> MSDTNYAVIYDLHSHTTASDGCLTPEALVHRAVEMRVGTLAITDHDTTAAIAPAREEISRSGLALNLIPGVEISTVWENHEIHIVGLNIDITHPLMCEFLAQQTERRNQRAQLIAERLEKAQIPGALEGAQRLAQGGAVTRGHFARFLVECGKASSMADVFKKYLARGKTGYVPPQWCTIEQAIDVIHHSGGKAVLAHPGRYNLSAKWLKRLVAHFAEHHGDAMEVAQCQQSPNERTQLAALARQHHLWASQGSDFHQPCPWIELGRKLWLPAGVEGVWQLWEQPQNTTEREL

RNase AM is so far the only 5′-3′ exoribonuclease known in E. coli, the enzymatic activity of which has been shown to be essential for the processing of bacterial ribosomal RNA. RNase AM belongs to the PHP domain family of proteins which is composed of amidohydrolases/phosphoesterases and is present in some DNA polymerases. To test this, we assessed the deFADding and deNADding activities of a recently characterized 5′-3′ exoribonuclease in E. coli, RNase AM (yciV), which can hydrolyze short RNAs of up to five nucleotides with a 5′P. We were able to expand on the original observations and demonstrate that a 40 nucleotide RNA molecule can also be degraded by RNase AM and further demonstrate the exonuclease activity is processive. Intriguingly, RNase AM also demonstrated robust deFADding activity, but unlike the two eukaryotic nucleases, RNase AM did not hydrolyze NAD-capped RNA.

To gain insight into how an exoribonuclease could function as a deFADding enzyme, we attempted to determine the crystal structure of E. coli RNase AM in complex with FAD in an effort to elucidate the mechanism for RNase AM monophosphate hydrolysis and deFADding activities. However, no crystals were obtained for RNase AM alone or in the presence of FAD. No density for the RNase AM insertion domain was observed, indicating that the domain is disordered in this crystal. The final structure consists of residues 9–106 and 177–284 and is modeled with three manganese ions (Mnα, Mnβ, and Mnγ) and a sulfate molecule in the active site. The refined atomic model contained no RNA and has excellent agreement with the X-ray diffraction data and the expected bond lengths, bond angles and other geometric parameters. RNase AM has a distorted (β/α)7-barrel fold and a three metal enzyme active site composed of histidines and aspartates/glutamate residues. Mnα and Mnβ, which are proposed to coordinate the water for nucleophilic attack are coordinated by residues His13, Glu72 and Asp255, and Glu72, His83 and His198 respectively. Mnγ is coordinated by residues Asp20, His45 and His257. The sulfate molecule coordinates all three metals and forms a salt bridge with Arg201, which may stabilize the hydrolysis reaction intermediate. Comparison to the CV1693 product complex containing AMP and Pi shows that RNase AM has the same overall fold and active site architecture, and the RNase AM sulfate is in the same position as the phosphate product.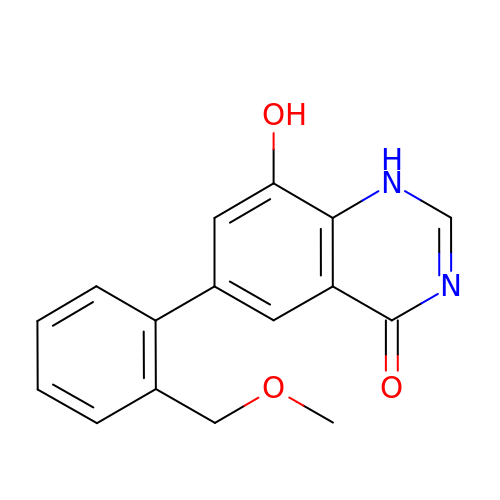6-[2-(methoxymethyl)phenyl]-8-oxidanyl-1~{H}-quinazolin-4-one | C16 H14 N2 O3 | CBWCDEQPQXXGLJ-UHFFFAOYSA-N>[3x]MIHLYDAKSFAKLRAAQYAAFHTDAPGSWFDHTSGVLESVEDGTPVLAIGVESGDAIVFDKNAQRIVAYKEKSVKAEDGSVSVVQVENGFMKQGHRGWLVDLTGELVGCSPVVAEFGGHRYASGMVIVTGKGNSGKTPLVHALGEALGGKD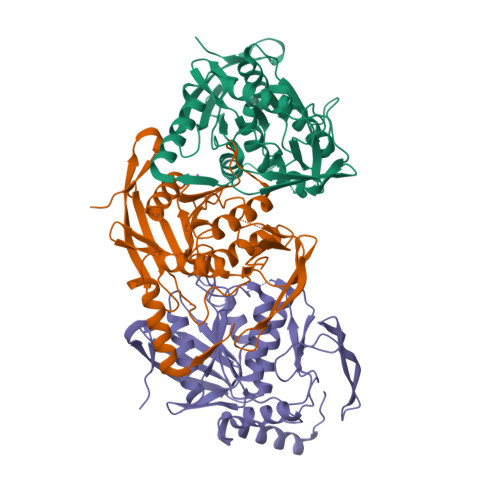KYATVRFGEPLSGYNTDFNVFVDDIARAMLQHRVIVIDSLKNVIGAAGGNTTSGGISRGAFDLLSDIGAMAASRGCVVIASLGPTSNDDKIVELVKEASRSNSTSLVISTDVDGEWQVLTRTGEGLQRLTHTLQTSYGEHSVLTIHTSKQSGGKQASGKAIQTVIKNDELESVLRRLTSN pmcMaackia amurensis seed lectin (MASL) is a plant lectin isolated from seeds of the M. amurensis tree. MASL has a strong affinity for sulfated carbohydrates and α2-3–linked sialic acids. Consequentially MASL is utilized as an agent to identify these residues on various proteins. Maackia amurensis lectins, including MASL, MAA, and MAL2, are widely utilized in biochemical and medicinal research.

Here, we present a high-resolution cryo-EM structure of MASL revealing that its tetrameric assembly is directed by two intersubunit disulfide bridges. However, the cryo-EM structure reveals additional stabilizing interactions within the MASL tetramer including hydrogen bonds between residues T210 and Q221, as well as between the carbonyl group of Q221 and K186 residues, which further stabilize the canonical dimer interface and prevent its dissociation. Each monomer harbors a calcium and manganese ion located within the external loops, resulting in the tetrameric protein structure harboring a total of four calcium and four manganese atoms, as shown in Figure 2, A and B. A structural comparison between previously reported substrate-bound MASL and the apo form of the lectin obtained in this study shows that the overall rotameric positions of the carbohydrate-binding site residues remain largely unchanged (RMSD = 0.56 Å). However, in the apo form, the Y250 residue is rotated approximately 90 degrees, closing the carbohydrate-binding cavity and creating a steric clash with the position of sialyllactose observed in a substrate-bound MASL as shown in Figure 5, A and B. The flipping of Y250 is presumed to occur as part of an induced fit mechanism, in which the binding pocket reshapes itself to enhance molecular recognition.

>[4x]MATSNSKPTQVLLATFLTFFFLLLNNVNSSDELSFTINNFVPNEADLLFQGEASVSSTGVLQLTRVENGQPQQYSVGRALYAAPVRIWDNTTGSVASFSTSFTFVVKAPNPDITSDGLAFYLAPPDSQIPSGSVSKYLGLFNNSNSDSSNQIVAVEFDTYFGHSYDPWDPNYRHIGIDVNGIESIKTVQWDWINGGVAFATITYLAPNKTLIASLVYPSNQTTFSVAASVDLKEILPEWVRVGFSAATGYPTEVETHDVLSWSFTSTLEANCDAATENNVHIARYTA>MGSDKIHHHHHHMKVVTFGEIMLRLSPPDHKRIFQTDSFDVTYGGAEANVAAFLAQMGLDAYFVTKLPNNPLGDAAAGHLRKFGVKTDYIARGGNRIGIYFLEIGASQRPSKVVYDRAHSAISEAKREDFDWEKILDGARWFHFSGITPPLGKELPLILEDALKVANEKGVTVSCDLNYRARLWTKEEAQKVMIPFMEYVDVLIANEEDIEKVLGISVEGLDLKTGKLNREAYAKIAEEVTRKYNFKTVGITLRESISATVNYWSVMVFENGQPHFSNRYEIHI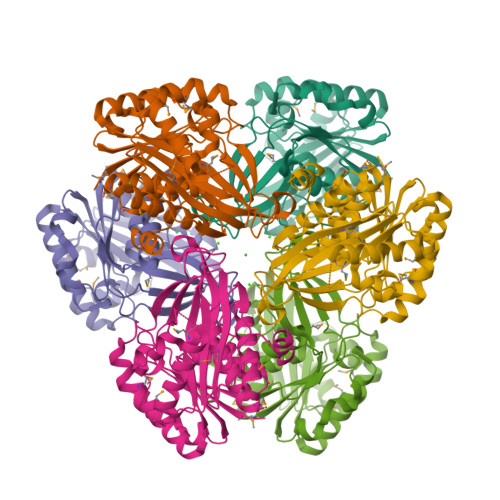VDRVGAGDSFAGALIYGSLMGFDSQKKAEFAAAASCLKHTIPGDFVVLSIEEIEKLASGATSGRVER[2x]>EPRSFEVGMLVWHKHKKYPFWPAVVKSVRQRDKKASVLYIEGHMNPKMKGFTVSLKSLKHFDCKEKQTLLNQAREDFNQDIGWCVSLITDYRVRLGCGSF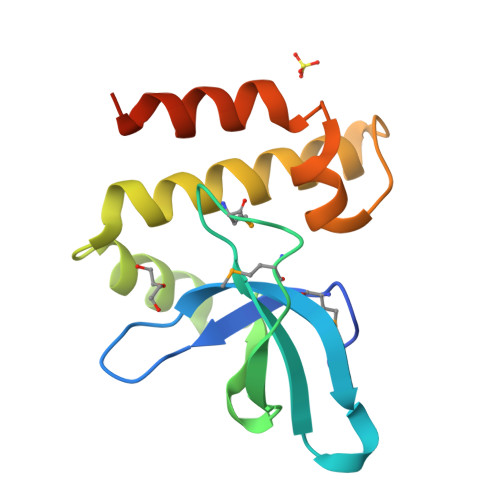AGSFLEYYAADISYPVRKSIQQDVLGTKLPQLSK[4x]>SAVKAARYGKDNVRVYKVHKDEKTGVQTVYEMTVCVLLEGEIETSYTKADNSVIVATDSIKNTIYITAKQNPVTPPELFGSILGTHFIEKYNHIHAAHVNIVCHRWTRMDIDGKPHPHSFIRDSEEKRNVQVDVVEGKGIDIKSSLSGLTVLKSTNSQFWGFLRDEYTTLKETWDRILSTDVDATWQWKNFSGLQEVRSHVPKFDATWATAREVTLKTFAEDNSASVQATMYKMAEQILARQQLIETVEYSLPNKHYFEIDLSWHKGLQNTGKNAEVFAPQ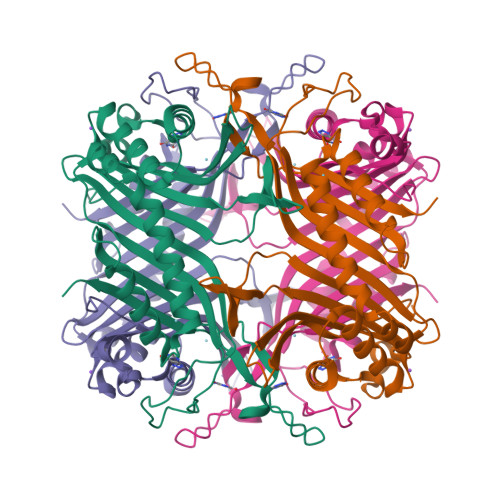SDPNGLIKCTVGRS[2x]>DARQRLKEVEVDDNGQFMTTDFGGNIEEQFSLKAGGRGSTLLEDFIFRQKLQHFDHERIPERVVHARGAGAHGIFTSYGDWSNITAASFLGAKDKQTPVFVRFSTVAGSRGSADTARDVHGFATRFYTDEGNFDIVGNNIPVFFIQDAIRFPDLIHSVKPSPDNEVPQAATAHDSAWDFFSSQPSALHTLFWAMSGNGIPRSYRHMDGFGIHTFRLVTEDGKSKLVKWHWKTKQGKAALVWEEAQVLAGKNADFHRQDLWDAIESGNAPSWELAVQLIDEDKAQAYGFDLLDPTKFLPEEFAPLQVLGEMTLNRNPMNYFAETEQISFQPGHIVRGVDFTEDPLLQGRLYSYLDTQLNRHRGPNFEQLPINRPVSGVHNNHRDGQGQAWIHKNIHHYSPSYLNKGYPAQANQTVGRGFFTTPGRTASGVLNRELSATFDDHYTQPRLFFNSLTPVEQQFVINAIRFEASHVTNEQVKKNVLEQLNKISNDVAKRVAVALGLEAPQPDPTYYHNNVTRGVSIFNESLPTIATLRVGVLSTTKGGSLDKAKALKEQLEKDGLKVTVIAEYLASGVDQTYSAADATAFDAVVVAEGAERVFSGKGAMSPLFPAGRPSQILTDGYRWGKPVAAVGSAKKALQSIGVEEKEAGVYAGAQDEVIKGVEEGLKVFK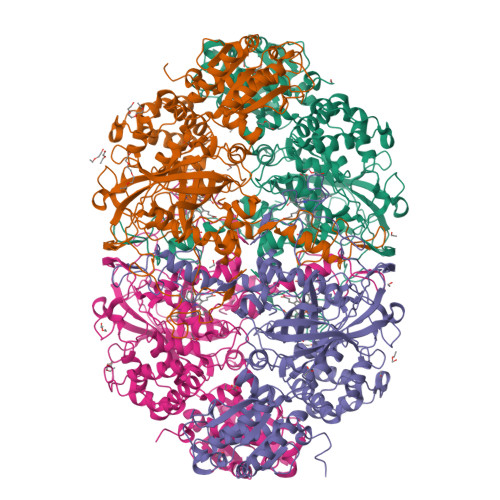FLERFAVDGDDEE[4x]As a core molecular machinery in mammalian autophagy, the ULK complex is composed of a serine–threonine ULK1/2 kinase, ATG13, ATG101, and FIP200 (also named as RB1CC1), and functions as a master regulator in the initiation of autophagy under the nutrient deprivation condition by linking the upstream nutrient sensors with the downstream autophagy machines. The ULK complex initiates the autophagosome formation, and has recently been implicated in selective autophagy by interacting with autophagy receptors through its FIP200 subunit. Here, we discover that the interactions of FIP200 Claw domain with autophagy receptors CCPG1 and Optineurin can be regulated by the phosphorylation in their respective FIP200-binding regions. In all, our findings uncover a general and phosphoregulatable binding mode shared by many autophagy receptors to interact with FIP200 Claw for autophagosome biogenesis, and are valuable for further understanding the molecular mechanism of selective autophagy.

To test this hypothesis, we quantitatively measured the interactions of FIP200 Claw (residue 1490–1594) with a 13-residue synthetic phospho-CCPG1 FIR2 peptide (“SDDpSDIVTLEPPK”, referred to as p-CCPG1 FIR2) and an un-phosphorylated CCPG1 FIR2 counterpart using fluorescence spectroscopy, and found the p-CCPG1 FIR2 binds to FIP200 Claw domain (residues 1490–1594) with a much stronger affinity compared with that of the wild-type CCPG1 FIR2. Fortunately, using the purified FIP200(1490–1594) mixed with excess amount of p-CCPG1 FIR2 peptide, we successfully obtained high-quality crystals and solved the FIP200 Claw/p-CCPG1 FIR2 complex structure at 1.40 Å resolution. In an asymmetric unit, there is only one FIP200 Claw molecule that is bound with a p-CCPG1 FIR2 peptide in a 1:1 stoichiometry. Further crystallographic symmetry analysis showed that the FIP200 Claw/p-CCPG1 FIR2 complex actually forms a symmetrical hetero-tetramer consisting of two p-CCPG1 FIR2 molecules and one FIP200 Claw dimer, in line with our analytical ultracentrifugation analysis. In the complex structure, the monomeric Claw domain of FIP200 adopts a unique architecture assembled by a 5-stranded anti-parallel β-sheet, a short α-helix, and a relatively isolated N-terminal β0-strand that directly packs with the counterpart β0-strand of another Claw monomer in an anti-parallel manner for the homo-dimerization of Claw. The clearly defined p-CCPG1 FIR2 in the complex structure contains 11 highly conserved residues (DpSDIVTLEPPK), and mainly forms a short β-strand that directly augments the C-terminal portion of the β4-strand of FIP200 Claw in an anti-parallel manner and at a location far away from the Claw dimerization interface. In the FIP200 Claw/p-CCPG1 FIR2 complex structure, the entire p-CCPG1 FIR2 packs extensively with a solvent-exposed concave groove formed by the β4 and β5 strands as well as the β4/β5 connecting loop that folds back to the β-sheet of FIP200 Claw, burying a total surface area of ~579 Å2.

> SRHSEKIAIRDFQVGDLVLIILDERHDNYVLFTVSPTLYFLHSESLPALDLKPGEGASGASRRPWVLGKVMEKEYCQAKKAQNRFKVPLGTKFYRVKAVSWNKKV;> SDDSDIVTLEPPK> MSTLANLTEVLFRLDFDPDTAVYHYRGQTLSRLQCRTYILSQASQLARLLKPGDRVVLALNDSPSLACLFLACIAVGAIPAVINPKSREQALADIAADCQASLVVREADAPSLSGPLAPLTLRAAAGRPLLDDFSLDALVGPADLDWSAFHRQDPAAACFLQYTSGSTGAPKGVMHSLRNTLGFCRAFATELLALQAGDRLYSIPKMFFGYGMGNSLFFPWFSGASALLDDTWPSPERVLENLVAFRPRVLFGVPAIYASLRPQARELLS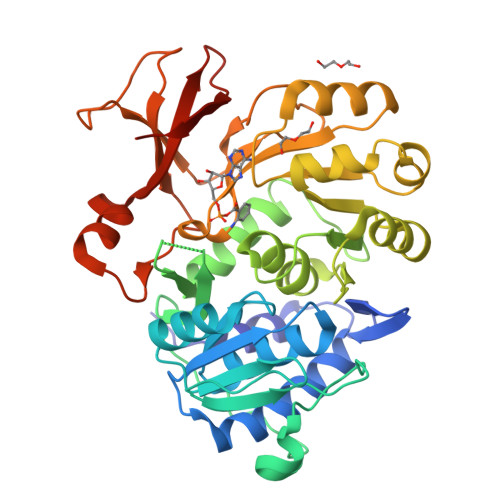SVRLAFSAGSPLPRGEFEFWAAHGLEICDGIGATEVGHVFLANRPGQARADSTGLPLPGYECRLVDREGHTIEEAGRQGVLLVRGPGLSPGYWRASEEQQARFAGGWYRTGDLFERDESGAYRHCGREDLEHHHHHH>MTSVTSKQSTILGSDEIDLGRVIGELIDHRKLIISITSVFTLFAILYALLATPIYETDALIQIEQKQGNAILSSLSQVLPDGQPQSAPETALLQSRMILGKTIDDLNLQIQIEQKYFPVIGRGLARLMGEKPGNIDITRLYLPDSDDISNNTPSIILTVKDKENYSINSDGIQLNGVVGTLLNEKGISLLVNEIDAKPGDQFVITQLPRLKAISDLLKSFSVADLGKDTGMLTLTLTGDNPKRISHILDSISQNYLAQNIARQAAQDAKSLEFLNQQLPKVRAELDSAEDKLNAYRKQKDSVDLNMEAKSVLDQIVNVDNQLNELTFREAEVSQLYTKEHPTYKALMEKRQTLQEEKSKLNKRVSSMPSTQQEVLRLSRDVESGRAVYLQLLNRQQELNIAKSSAIGNVRIIDNAVTDPNPVRPKKTIIIVIGVVLGLIVSVVLVLFQVFLRRGIESPEQLEEIGINVYASIPISEWLTKNARQSGKVRKNQSDTLLAVGNPADLAVEAIRGLRTSLHFAMMEAKNNVLMISGASPSAGMTFISSNLAATIAITGKKVLFIDADLRKGYAHKMFGHKNDKGLSEFLSGQAAAEMIIDKVEGGGFDYIGRGQIPPNPAELLMHPRFEQLLNWASQNYDLIIIDTPPILAVTDAAIIGRYAGTCLLVARFEKNTVKEIDVSMKRFEQSGVVVKGCILNGVVKKASSYYRYGHYHYGESEEDKKHHHHHH[8x]

Wzc, an integral cytoplasmic membrane tyrosine autokinase protein serves as the master regulator of the biosynthesis and export of many bacterial capsular polysaccharides and exopolysaccharides. Wzc comprises a large periplasmic domain, two transmembrane helices and a C-terminal cytoplasmic kinase domain with a tyrosine-rich tail. Wzc regulates polymerisation functions through cycling the formation and dissociation of an octameric complex, driven by changes in the phosphorylation status of the tyrosine-rich tail. E. coli Wzc serves a model for a wider family of polysaccharide co-polymerases.

Here, we report the characterisation of the structures WzcK540M2YE (Y718E, Y717E), WzcK540M3YE (Y718E, Y717E and Y715E) and WzcK540M3YE_N711Y (an additional N711Y mutation) corresponding to different phosphorylation states. One intermediate, 2pY which has Y713 at the active site, does not follow the YxY pattern, since position 711 is asparagine. We show that it is binding of the i-2 tyrosine to the tyrosine pocket (where i is the number of the residue positioned at the kinase active site) orders the tail between the tyrosine at the active site and helix α23. A mutant of 2pY (Wzc3YE_N711Y) stabilises the C-terminal tail was functional in vivo, restoring immunoreactive CPS to levels approximating the wild type. This is consistent with a model in which the more stable the Wzc octamer the higher the Wzy activity. We note the reduction of CPS production by destabilising D28A and K701A mutants further support this model. The Wzc3YE_N711Y shows greater phosphorylation relative to Wzc3YE and proteomic analysis of purified WzcYF_713Y/N711Y reveals both N711Y and Y713 are phosphorylated. We propose that the YxY pattern serves as a molecular ratchet, that by selecting a tyrosine over phosphotyrosine, ensures phosphorylations in unidirectional (moving from the C to the N).In siphophage T5, the unique RBP is located at the extremity of a central fiber. FhuA, an outer membrane E. coli iron-ferrichrome transporter, is the bacterial receptor recognized by T5 (25). We present the structures of T5 tail tip, determined by cryo–electron microscopy before and after interaction with its E. coli receptor, FhuA, reconstituted into nanodisc. These structures bring out the important conformational changes undergone by T5 tail tip upon infection, which include bending of T5 central fiber on the side of the tail tip, tail anchoring to the membrane, tail tube opening, and formation of a transmembrane channel.

(H) Cryo-EM structure of Tip-FhuA at resolutions ranging from 3.6- to 4.3-Å resolution. Upon RBPpb5 binding to FhuA, the central fiber reorganizes: The three FNIIIs strings dissociate, two strings relocate on one side of BHPpb3, and the third one on the other side. The central fiber bends by ~160° at the level of the hinge between the third pb4 FNIII and pb4 spike: The latter is now surrounded and stabilized by pb4 FNIIIs, which interact with and stabilize pb4 spike small decoration domains. pb4 spike also undergoes structural rearrangement, with a different twist of the spike. This bending and stabilization of the central fiber bring the tail tube closer to the membrane, orient it correctly, and anchor the tail to the membrane. To accommodate for the drastic conformational changes of the FNIII strings induced by the bending of the central fiber, BHPpb3 hdIV-FNIII linker is pulled and, like a zip, disrupts the interaction network between neighboring BHPpb3 monomers and with BHPpb3 plug. This then allows the rotation of BHPpb3 hdII-III, plug unfolding/refolding, opening of the tube, and anchoring of BHPpb3 to the membrane via the β-hairpin legs. The three β-hairpin legs connect BHPpb3 to the nanodisc: Their tip is composed of 233-Leu-Phe-Gly-Leu-236, which would insert into the outer leaflet of the lipid bilayer hydrophobic core. In the crevice opened at the interface between two BHPpb3 subunits, extra densities were identified, in which the 43 C-terminal residues of TMPpb2* could be modeled. Thus, T5 tail tube is anchored to the outer membrane by both BHPpb3 and TMPpb2*, in addition to FhuA-RBPpb5: It ensures that the tail tube is locked in register with the channel formed by TMPpb2* in the outer membrane. At low contour level, aligned with the tail tube lumen, a hole in the nanodisc is observed, strongly suggesting the presence of a channel at this position.

>[6x]MSLQLLRNTRIFVSTVKTGHNKTNTQEILVQDDISWGQDSNSTDITVNEAGPRPTRGSKRFNDSLNAAEWSFSTYILPYKDKNTSKQIVPDYMLWHALSSGRAINLEGTTGAHNNATNFMVNFKDNSYHELAMLHIYILTDKTWSYIDSCQINQAEVNVDIEDIGRVTWSGNGNQLIPLDEQPFDPDQIGIDDETYMTIQGSYIKNKLTILKIKDMDTNKSYDIPITGGTFTINNNITYLTPNVMSRVTIPIGSFTGAFELTGSLTAYLNDKSLGSMELYKDLIKTLKVVNRFEIALVLGGEYDDERPAAILVAKQAHVNIPTIETDDVLGTSVEFKAIPSDLDAGDEGYLGFSSKYTRTTINNLIVNGDGATDAVTAITVKSAGNVTTLNRSATLQMSVEVTPSSARNKEVTWAITAGDAATINATGLLRADASKTGAVTVEATAKDGSGVKGTKVITVTAGG;>[3x]MFYSLMRESKIVIEYDGRGYHFDALSNYDASTSFQEFKTLRRTIHNRTNYADSIINAQDPSSISLAINFSTTLIESNFFDWMGFTREGNSLFLPRNTPNIEPIMFNMYIINHNNSCIYFENCYVSTVDFSLDKSIPILNVGIESGKFSEVSTFRDGYTITQGEVLPYSAPAVYTNSSPLPALISASMSFQQQCSWREDRNIFDINKIYTNKRAYVNEMNASATLAFYYVKRLVGDKFLNLDPETRTPLIIKNKYVSITFPLARISKRLNFSDLYQVEYDVIPTADSDPVEINFFGERK;>[12x]MSTENRVIDLVVDENVPYGLLMQFMDVDDSVYPSTSKPVDLTDFSLRGSIKSSLEDGAETVASFTTAIVDAAQGVASISLPVSAVTTIASKASKERDRYNPRQRLAGYYDVIITRTAVGSAASSFRIMEGKVYISDGVTQ;>MRLPDPYTNPEYPGLGFESVNLVDNDPMIRDELPNGKVKEVKISAQYWGINISYPELFPDEYAFLDSRLLEYKRTGDYLDVLLPQYEAFRVRGDTKSVTIPAGQKGSQIILNTNGTLTGQPKAGDLFKLSTHPKVYKITNFSSSGNVWNISLYPDLFITTTGSEKPVFNGILFRTKLMNGDSFGSTLNNNGTYSGISLSLRESL[6x];>[3x]MKKILDSAKNYLNTHDKLKTACLIALELPSSSGSAATYIYLTDYFRDVTYNGILYRSGKVKSISSHKQNRQLSIGSLSFTITGTAEDEVLKLVQNGVSFLDRGITIHQAIINEEGNILPVDPDTDGPLLFFRGRITGGGIKDNVNTSGIGTSVITWNCSNQFYDFDRVNGRYTDDASHRGLEVVNGTLQPSNGAKRPEYQEDYGFFHSNKSTTILAKYQVKEERYKLQSKKKLFGLSRSYSLKKYYETVTKEVDLDFNLAAKFIPVVYGVQKIPGIPIFADTELNNPNIVYVVYAFAEGEIDGFLDFYIGDSPMICFDETDSDTRTCFGRKKIVGDTMHRLAAGTSTSQPSVHGQEYKYNDGNGDIRIWTFHGKPDQTAAQVLVDIAKKKGFYLQNQNGNGPEYWDSRYKLLDTAYAIVRFTINENRTEIPEISAEVQGKKVKVYNSDGTIKADKTSLNGIWQLMDYLTSDRYGADITLDQFPLQKVISEAKILDIIDESYQTSWQPYWRYVGWNDPLSENRQIVQLNTILDTSESVFKNVQGILESFGGAINNLSGEYRITVEKYSTNPLRINFLDTYGDLDLSDTTGRNKFNSVQASLVDPALSWKTNSITFYNSKFKEQDKGLDKKLQLSFANITNYYTARSYADRELKKSRYSRTLSFSVPYKFIGIEPNDPIAFTYERYGWKDKFFLVDEVENTRDGKINLVLQEYGEDVFINSEQVDNSGNDIPDISNNVLPPRDFKYTPTPGGVVGAIGKNGELSWLPSLTNNVVYYSIAHSGHVNPYIVQQLENNPNERMIQEIIGEPAGLAIFELRAVDINGRRSSPVTLSVDLNSAKNLSVVSNFRVVNTASGDVTEFVGPDVKLAWDKIPEEEIIPEIYYTLEIYDSQDRMLRSVRIEDVYTYDYLLTYNKADFALLNSGALGINRKLRFRIRAEGENGEQSVGWATI;>MISNNAPAKMVLNSVLTGYTLAYIQHSIYSDYDVIGRSFWLKEGSNVTRRDFTGIDTFSVTINNLKPTTTYEVQGAFYDSIIDSELLNAQIGINLSDKQTFKMKSAPRITGARCESEPVDVGVGAPIVYIDTTGEADYCTIELKDNSNANNPWVKYYVGALMPTIMFGGVPIGSYKVRISGQISLPDGVTIDSSGYYEYPNVFEVRYNFVPPAAPINIVFKAARIADGKERYDLRVQWDWNRGAGANVREFVLSYIDSAEFVRTGWTKAQKINVGAAQSATIISFPWKVEHKFKVSSIAWGPDAQDVTDSAVQTFILNESTPLDNSFVNETGIEVNYAYIKGKIKDGSTWKQTFLIDAATGAINIGLLDAEGKAPISFDPVKKIVNVDGSVITKTINAANFVMTNLTGQDNPAIYTQGKTWGDTKSGIWMGMDNVTAKPKLDIGNATQYIRYDGNILRISSEVVIGTPNGDIDIQTGIQGKQTVFIYIIGTSLPAKPTSPAYPPSGWSKTPPNRTSNTQNIYCSTGTLDPVTNQLVSGTSWSDVVQWSGTEGVDGRPGATGQRGPGMYSLAIANLTAWNDSQANSFFTSNFGSGPVKYDVLTEYKSGAPGTAFTRQWNGSAWTSPAMVLHGDMIVNGTVTASKIVANNAFLSQIGVNIIYDRAAALSSNPEGSYKMKIDLQNGYIHIR[3x];>MTDKLIRELLIDVKQKGATRTAKSIENVSDALENAAAASELTNEQLGKMPRTLYSIERAADRAAKSLTKMQASRGMAGITKSIDGIGDKLDYLAIQLIEVTDKLEIGFDGVSRSVKAMGNDVAAATEKVQDRLYDTNRALGGTSKGFNDTAGAAGRASRALGNTSGSARGATRDFAAMAKIGGRLPIMYAALASNVFVLQTAFESLKVGDQLNRLEQFGTIVGTMTGTPVQTLALSLQNATNGAISFEEAMRQASSASAYGFDSEQLEQFGLVARRAAAVLGVDMTDALNRVIKGVSKQEIELLDELGVTIRLNDAYENYVKQLNATSTGIKYTVDSLTTYQKQQAYANEVIAESTRRFGYLDDALKATSWEQFAANANSALRSLQQSAATYLNPVMDTLNTFLYQTKSSQMRVSAMARSASAKTTPAENVTALIENAVGAREDLDTYLKESEERVKKAQELKQQLDDLKAKQAATAPIANALTAGGIGGDESNKLVVQLTNELARQNKEIEERTKTEKVLRQAVQDTGEALLRNGKLAEQLGAKMKYADTAVPGDKGVFEVDPNNLKAVSEIQKNFDFLKKSSSDTANNIRMAASSITNAKKASSDLNSVVKAVEDTSKVTGQSADTLVKNLNLGFSSLDQMKAAQKGLSEYVTAMDKSEQNALEVAKRKDEVYNQTKDKAKAEAAAREVLLRQQQEQLTAAKALLAINPNDPEALKQVAKIETEILNTKAQGFENAKKTKDYTDKILGVDREIALLNDRTMTSTQYRLAQLRLELQLEQEKTELYSKQADGQAKVEQSRRAQAQISREIWEAEKQGTASHVSALMDALEVSQTQRNVTGQSQILTERLSILQQQLELSKGNTEEELKYRNEIYKTSAALEQLKKQRESQMQQQVGSSVGATYTSTTGLIGEDKDFADMQNRMASYDQAISKLSELNSEATAVAQSMGNLTNAMIQFSQGSLDTTSMIASGMQTVASMIQYSTSQQVSAIDQAIAAEQKRDGKSEASKAKLKKLEAEKLKIQQDAAKKQIIIQTAVAVMQAATAVPYPFSIPLMVAAGLAGALALAQASSASGMSSIADSGADTTQYLTLGERQKNVDVSMQASSGELSYLRGDKGIGNANSFVPRAEGGMMYPGVSYQMGEHGTEVVTPMVPMKATPNDQLSDGSKTTSGRPIILNISTMDAASFRDFASNNSTAFRDAVELALNENGTTLKSLGNS[3x]>[8x]MTSVTSKQSTILGSDEIDLGRVIGELIDHRKLIISITSVFTLFAILYALLATPIYETDALIQIEQKQGNAILSSLSQVLPDGQPQSAPETALLQSRMILGKTIDDLNLQIQIEQKYFPVIGRGLARLMGEKPGNIDITRLYLPDSDDISNNTPSIILTVKDKENYSINSDGIQLNGVVGTLLNEKGISLLVNEIDAKPGDQFVIT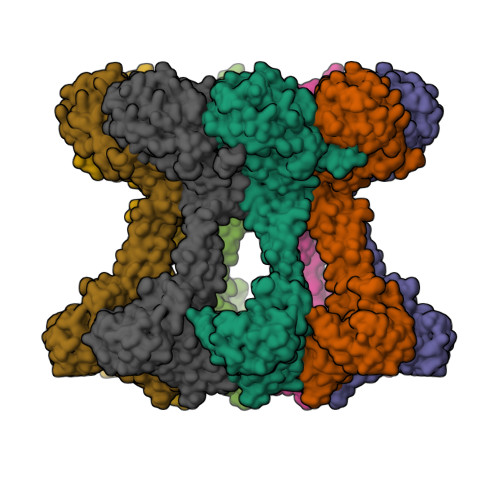QLPRLKAISDLLKSFSVADLGKDTGMLTLTLTGDNPKRISHILDSISQNYLAQNIARQAAQDAKSLEFLNQQLPKVRAELDSAEDKLNAYRKQKDSVDLNMEAKSVLDQIVNVDNQLNELTFREAEVSQLYTKEHPTYKALMEKRQTLQEEKSKLNKRVSSMPSTQQEVLRLSRDVESGRAVYLQLLNRQQELNIAKSSAIGNVRIIDNAVTDPNPVRPKKTIIIVIGVVLGLIVSVVLVLFQVFLRRGIESPEQLEEIGINVYASIPISEWLTKNARQSGKVRKNQSDTLLAVGNPADLAVEAIRGLRTSLHFAMMEAKNNVLMISGASPSAGMTFISSNLAATIAITGKKVLFIDADLRKGYAHKMFGHKNDKGLSEFLSGQAAAEMIIDKVEGGGFDYIGRGQIPPNPAELLMHPRFEQLLNWASQNYDLIIIDTPPILAVTDAAIIGRYAGTCLLVARFEKNTVKEIDVSMKRFEQSGVVVKGCILNGVVKKASSYYRYGHNHYGYSYYDKKHHHHHH1-(4-{4-[7-amino-2-(1,2,3-benzothiadiazol-7-yl)furo[2,3-c]pyridin-4-yl]-1H-pyrazol-1-yl}piperidin-1-yl)ethanone | C23 H21 N7 O2 S | 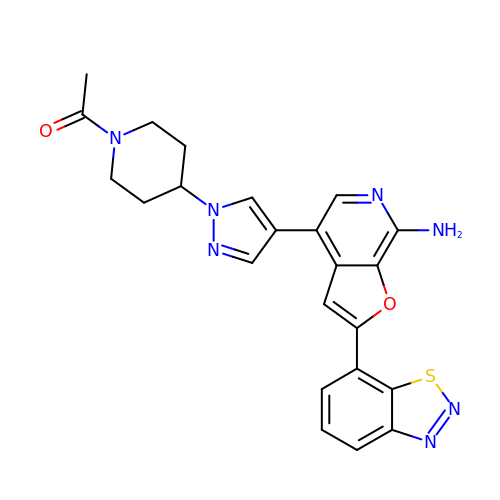XDCWLOMVUOZXFY-UHFFFAOYSA-N>[4x]SHSEEPAEILPPARDEEEEEEEGMEQGLEEEEEVDPRIQGELEKLNQSTDDINRRETELEDARQKFRSVLVEATVKLDELVKKIGKAVEDSKPYWEARRVARQAQLEAQKATQDFQRATEVLRAAKETISLAEQRLLEDDKRQFDSAWQEMLNHATQRVMEAEQTKTRSELVHKETAARYNAAMGRMRQLEKKLKRAINKSKPYFELKAKYYVQLEQLKKTVDDLQAKLTLAKGEYKMALKNLEMISDEIHERRRSSAMGPRGCGVGAE;>SHMGTRDDEYDYLFKVVLIGDSGVGKSNLLSRFTRNEFNLESKSTIGVEFATRSIQVDGKTIKAQIWDTAGQERYRAITSAYYRGAVGALLVYDIAKHLTYENVERWLKELRDHADSNIVIMLVGNKSDLRHLRAVPTDEARAFAEKNGLSFIETSALDSTNVEAAFQTILTEIY[4x]

The Rab11 subfamily plays important roles in specific trafficking events such as exocytosis, endosomal recycling, and cytokinesis. SH3BP5 and SH3BP5-like (SH3BP5L) proteins have recently been found to serve as guanine nucleotide exchange factors (GEF) for Rab11. SH3BP5 exhibits a V-shaped structure comprising two coiled coils. The coiled coil composed of α1, and α4 is solely responsible for the Rab11a binding and GEF activity.

To elucidate the GEF mechanism of SH3BP5, we also determined the crystal structure of SH3BP5 in the complex with Rab11a at 3.8 Å resolution. Wild-type SH3BP5 (10–276) was used for crystallization of the complex because SH3BP5-RA tended to crystallize in the apo form. The asymmetric unit contains four complexes, where SH3BP5 interacts with Rab11a in a similar manner. The electron density corresponding to the N- and C-terminal regions of SH3BP5 (residues 10–41 and 268–276, respectively) and the N-terminal four residues of Rab11a were invisible, suggesting the structural disorder of these regions. In the SH3BP5–Rab11a complex, both switch regions (switch I and switch II) of Rab11a interact with the coiled coil comprising α1 and α4 of SH3BP5. As compared with the GTP- or GDP-bound Rab11a structures, the switch I region is pulled out by SH3BP5 so as to facilitate the release of the bound guanine nucleotide and Mg2+ (21). The switch II region adopts a helical structure, which is also observed in the inactive, GDP-bound state of Rab11a. In summary, SH3BP5 opens the guanine nucleotide-binding pocket by capturing both switch regions. On the other hand, the P loop region, which binds to β- and γ-phosphate groups, does not contact SH3BP5 and remains folded as in the GDP- and GTP-bound structures. SH3BP5 interacts with the N-terminal region, interswitch, switch I, and switch II of Rab11a in the SH3BP5–Rab11a complex.>[3x]EAEAGSVASLRQQVEALQGQVQHLQAAFSQYKKVELFPNGQSVGEKIFKTAGFVKPFTEAQLLCTQAGGQLASP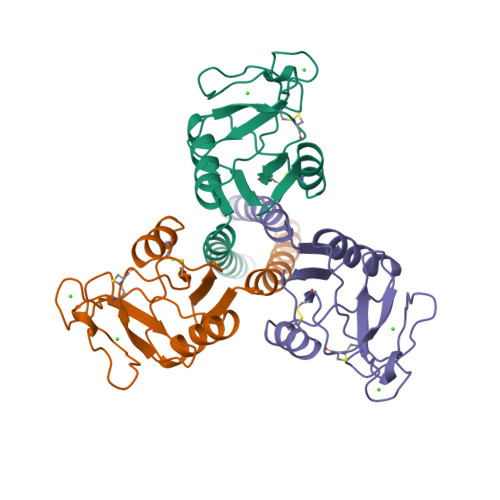RSAAENAALQQLVVAKNEAAFLSMTDSKTEGKFTYPTGESLVYSNWAPGEPNDDGGSEDCVEIFTNGKWNDRACGEKRLVVCEF>MGVHTFEEESTSPVPPAKLFKATVVDGDELTPKLIPAIQSIEIVEGNGGPGTVKKVTAVEDGKTSYVLHKIDAIDEATYTYDYTISGGTGFQEILEKVSFKTKLEAADGGSKIKVSVTFHTKG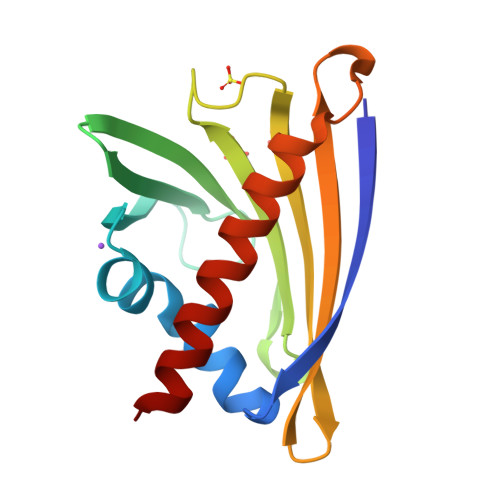DAPLPDEVHQDVKQKSQGIFKAIEGYVLSN[4x]> ADPLLLYANRRDLRLVDATNGKENATIVVGGLEDAAAVDFVFSHGLIYWSDVSEEAIKRTEFNKTESVQNVVVSGLLSPDGLACDWLGEKLYWTDSETNRIEVSNLDGSLRKVLFWQELDQPRAIALDPSSGFMYWTDWGEVPKIERAGMDGSSRFIIINSEIYWPNGLTLDYEEQKLYWADAKLNFIHKSNLDGTNRQAVVKGSLPHPFALTLFEDILYWTDWSTHSILACNKYTGEGLREIHSDIFSPMDIHAFSQQRQPNATNPCGIDNGGCSHLCLMSPVKPFYQCACPTGVKLLENGKTCKDGATELLLLARRTDLRRISLDTPDFTDIVLQLEDIRHAIAIDYDPVEGYIYWTDDEVRAIRRSFIDGSGSQFVVTAQIAHPDGIAVDWVARNLYWTDTGTDRIEVTRLNGTMRKILISEDLEEPR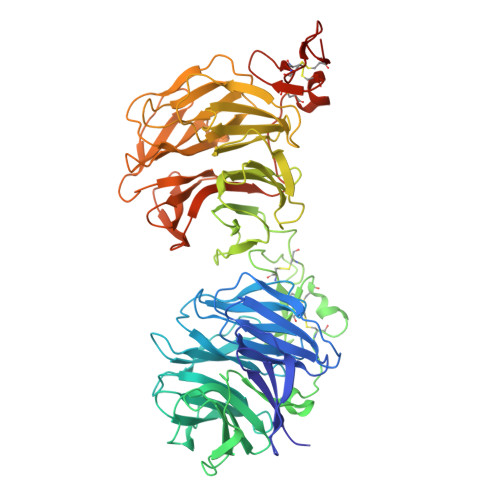AIVLDPMVGYMYWTDWGEIPKIERAALDGSDRVVLVNTSLGWPNGLALDYDEGKIYWGDAKTDKIEVMNTDGTGRRVLVEDKIPHIFGFTLLGDYVYWTDWQRRSIERVHKRSAEREVIIDQLPDLMGLKATNVHRVIGSNPCAEENGGCSHLCLYRPQGLRCACPIGFELISDMKTCIVPHHHHHHHHHH>MRSRRVDVMDVMNRLILAMDLMNRDDALRVTGEVREYIDTVKIGYPLVLSEGMDIIAEFRKRFGCRIIAGFKVADIPETNEKICRATFKAGADAIIVHGFPGADSVRACLNVAEEMGREVFLLTEMSHPGA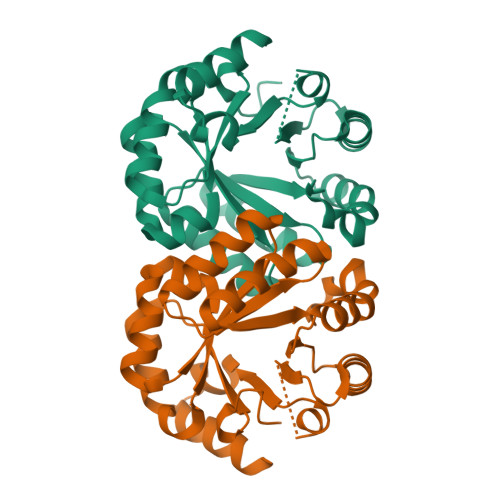EMFIQGAADEIARMGVDLGVKNYVGPSTRPERLSRLREIIGQDSFLISPGVGAQGGDPGETLRFADAIIVGRSIYLADNPAAAAAGIIESIKDLLNP[2x]Among the few candidates, the alcohol dehydrogenase from Thauera aromatica (ThaADH) stands out with a high activity for the reduction of the cyclic α‐diketone 1,2‐cyclohexanedione to the corresponding α‐hydroxy ketone. The results obtained confirm the previously observed preference of ThaADH for cyclic carbonyl compounds over aromatic and linear aliphatic compounds. This preference is in line with the physiological function of the enzyme, i. e. the oxidation of the cyclic 6‐hydroxycyclohex‐1‐ene‐1‐carboxyl‐CoA within the benzoyl‐CoA metabolism. The overall structural fold of ThaADH was consistent with those of many other MDR−ADHs, i. e. contains the typical C‐terminal coenzyme binding domain and N‐terminal catalytic domain. ThaADH shares with many ADHs of the MDR family the presence of two zinc atoms per monomer.

In this context, we determined the X‐ray crystallographic structure of the wild type (WT) ThaADH in complex with NADH, refined to a resolution of 2.60 Å, as well as of the double mutant K319A/K320A without cofactor, refined to 1.80 Å. In order to shed further light on structural features, the crystal structure of ThaADH was solved in two forms: First, the WT enzyme in complex with NADH, which had 3 molecules in the asymmetric unit (asu), comprising one‐and‐a‐half dimers, and was refined to a resolution of 2.60 Å. The quality of the model was good in monomers A and B but electron density was poorer for monomer C leading to some unmodelled side chains and higher B factors for this molecule. Analysis of the wild‐type structure using PISA supports the experimental data in suggesting a dimer as the majority oligomeric species in solution. Analysis using PISA suggested that the dimer interface of ThaADH has a salt bridge more than in CPCR2 (PDB 4 C4O) as a less stable related ADH. Residues coordinating the catalytic zinc in ThaADH are C42, H65, D156 and E66, but superposing ThaADH and CPCR2 structure suggests that the catalytic zinc of ThaADH is in a resting state as already described for CPCR2. For this reason, molecular docking of substrate molecules into the active site of ThaADH was omitted in this study, and 1,2‐cyclohexanedione was placed manually in the active site. To approximate a productive substrate binding, the maximum distance between the C4 atom of the nicotinamide ring of NADH and the carbonyl carbon of the carbonyl function (<3.2 Å) as well as the distance between the terminal carbonyl oxygen of substrate and the side chain of T44 as proton donor (<3 Å) were taken into account. Thus 1,2‐cyclohexanedione was placed in the active site of ThaADH with 3.0 Å and 2.7 Å distance between the atoms mentioned above, respectively. However, due to the manual placement of the substrate molecule without considering the catalytic zinc, the following models should be treated with caution.

>MSSNPHRWMMTSPGAPMVRAEFEIGELSADQVVVAVAGCGVCHTDLGYYYDSVRTNHALPLALGHEISGRVVQAGANAAQWLGRAVIVPAVMPCGTCELCTSGHGTICRDQVMPGNDIQGGFASHVVVPARGLCPVDEARLAAAGLQLADVSVVADAVTTPYQAVLQAGVEPGDVAVVIGVGGVGGYAVQIANAFGASVVAIDVDPAKLEMMSKHGAALTLNAREISGRDLKKAIEAHAKANGLRLTRWKIFECSGTGAGQTSAYGLLTHGATLAVVGFTMDKVEVRLSNLMAFHARALGNWGCLPEYYPAALDLVLDKKIDLASFIERHPLDQIGEVFAAAHAHKLTRRAILT[3x]>EVKQENRLLNESESSSQGLLGYYFSDLNFQAPMVVTSSTTGDLSIPSSELENIPSENQYFQSAIWSGFIKVKKSDEYTFATSADNHVTMWVDDQEVINKASNSNKIRLEKGRLYQIKIQYQRENPTEKGLDFKLYWTDSQNKKEVISSDNLQLPELKQKSSNSRKKRSTSAGPTVPDRDNDGIPDSLEVEGYTVDVKNKRTFLSPWISNIHEKKGLTKYKSSPEKWSTASDPYSDFEKVTGRIDKNVSPEARHPLVAAYPIVHVDMENIILSKNEDQSTQNTDSQTRTISKNTSTSRTHTSEVHGNAEVHASFFDIGGSVSAGFSNSNSSTVAIDHSLSLAGERTWAETMGLNTADTARLNANIRYVNTGTAPIYNVLPTTSLVLGKNQTLATIKAKENQLSQILAPNNYYPSKNLAPIALNAQDDFSSTPITMNYNQFLELEKTKQLRLDTDQVYGNIATYNFENGRVRVDTGSNWSEVLPQIQETTARIIFNGKDLNLVERRIAAVNPSDPLETTKPDMTLKEALKIAFGFNEPNGNLQYQGKDITEFDFNFDQQTSQNIKNQLAELNATNIYTVLDKIKLNAKMNILIRDKRFHYDRNNIAVGADESVVKEAHREVINSSTEGLLLNIDKDIRKILSGYIVEIEDTEGLKEVINDRYDMLNISSLRQDGKTFIDFKKYND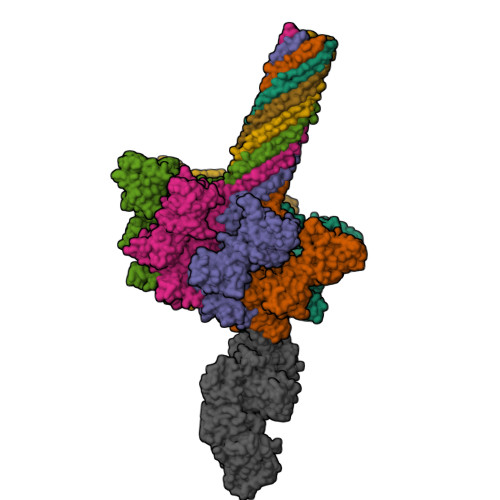KLPLYISNPNYKVNVYAVTKENTIINPSENGDTSTNGIKKILIFSKKGYEIG[7x];> MNEHYTESDIKRNHKTEKNKTEKEKFKDSINNLVKTEFTNETLDKIQQTQDLLKKIPKDVLEIYSELGGEIYFTDIDLVEHKELQDLSEEEKNSMNSRGEKVPFASRFVFEKKRETPKLIINIKDYAINSEQSKEVYYEIGKGISLDIISKDKSLDPEFLNLIKSLSDDSDSSDLLFSQKFKEKLELNNKSIDINFIKENLTEFQHAFSLAFSYYFAPDHRTVLELYAPDMFEYMNKLEKGGFEKISESLKKEGVEKDRIDVLKGEKALKASGLVPEHADAFKKIARELNTYILFRPVNKLATNLIKSGVATKGLNVHGKSSDWGPVAGYIPFDQDLSKKHGQQLAVEKGNLENKKSITEHEGEIGKIPLKLDHLRIEELKENGIILKGKKEIDNGKKYYLLESNNQVYEFRISDENNEVQYKTKEGKITVLGEKFNWRNIEVMAKNVEGVLKPLTADYDLFALAPSLTEIKKQIPQKEWDKVVNTPNSLEKQKGVTNLLIKYGIERKPDSTKGTLSNWQKQMLDRLNEAVKYTGYTGGDVVNHGTEQDNEEFPEKDNEIFIINPEGEFILTKNWEMTGRFIEKNITGKDYLYYFNRSYNKIAPGNKAYIEWTDPITKAKINTIPTSAEFIKNLSSIRRSSNVGVYKDSGDKDEFAKKESVKKIAGYLSDYYNSANHIFSQEKKRKISIFRGIQAYNEIENVLKSKQIAPEYKNYFQYLKERITNQVQLLLTHQKSNIEFKLLYKQLNFTENETDNFEVFQKIIDEK>[2x]NLKPVDAMQCFDCHTQIEDMHTVGKHATVNCVHCHDATEHVETASSRRMGERPVTRMDLEACATCHTAQFNSFVEVRHESHPRLEKATPTSRSPMFDKLIAGHGFAFEHAEPRSHAFMLVDHFVVDRAYGGRFQFKNWQKVTDGMGAVRGAWTVLTDADPESSDQRRFLSQTATAANPVCLNCKTQDHILDWAYMGDEHEAAKWSRTSEVVEFARDLNHPLNCFMCHDPHSAGPRVVRDGLINAVVDRGLGTYPHDPVKSEQQGMTKVTFQRGREDFRAIGLLDTADSNVMCAQCHVEYNCNPGYQLSDGSRVGMDDRRANHFFWANVFDYKEAAQEIDFFDFRHATTGAA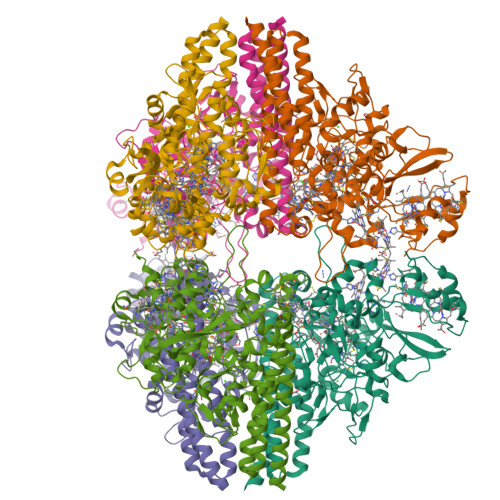LPKLQHPEAETFWGSVHERNGVACADCHMPKVQLENGKVYTSHSQRTPRDMMGQACLNCHAEWTEDQALYAIDYIKNYTHGKIVKSEYWLAKMIDLFPVAKRAGVSEDVLNQARELHYDAHLYWEWWTAENSVGFHNPDQARESLMTSISKSKEAVSLLNDAIDAQVA> DCPDGWSSTKSYCYRPFKEKKTWEEAERFCTEQEKEAHLVSMENRLEAVFVDMVMENNFENKIYRSWIGLKIENKGQRSNLEWSDGSSISYENLYEPYM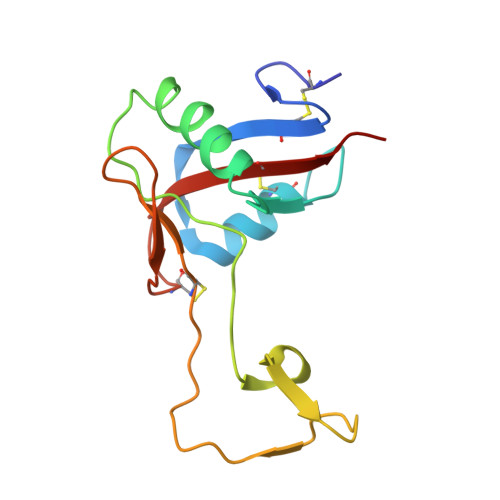EKCFLMDHQSGLPKWHTADCEEKNVFMCKFQLPR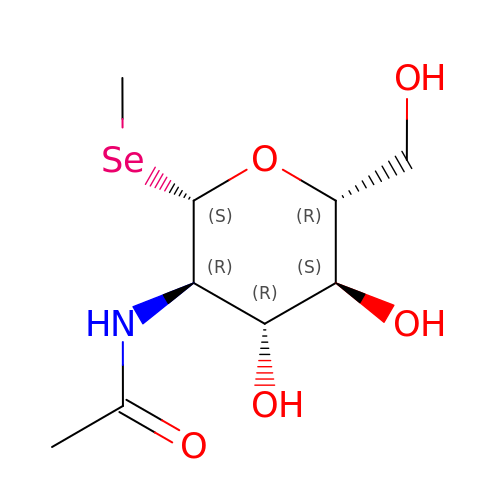methyl 2-acetamido-2-deoxy-1-seleno-beta-D-glucopyranoside | C9 H17 N O5 Se | AZZZNYGPGINRNT-OKNNCHMLSA-N> MPFVNKQFNYKDPVNGVDIAYIKIPNAGQMQPVKAFKIHNKIWVIPERDTFTNPEEGDLNPPPEAKQVPVSYYDSTYLSTDNEKDNYLKGVTKLFERIYSTDLGRMLLTSIVRGIPFWGGSTIDTELKVIDTNCINVIQPDGSYRSEELNLVIIGPSADIIQFECKSFGHEVLNLTRNGYGSTQYIRFSPDFTFGFEESLEVDTNPLLGAGKFATDPAVTLAHQLIHAGHRLYGIAINPNRVFKVNTNAYYEMSGLEVSFEELRTFGGHDAKFIDSLQENEFRLYYYNKFKDIASTLNKAKSIVGTTASLQYMKNVFKEKYLLSEDTSGKFSVDKLKFDKLYKMLTEIYTEDNFVKFFKVLNAKTFLNFDKAVFKINIVPKVNYTIYDGFNLRNTNLAANFNGQNTEINNMNFTKLKNFTGLFEFYKLLCVRGIITSKTKSLDKGYNKALNDLCIKVNNWDLFFSPSEDNFTNDLNKGEEITSDTNIEAAEENISLDLIQQYYLTFNFDNEPENISIENLSSDIIGQLELMPNIERFPNGKKYELDKYTMFHYLRAQEFEHGKSRIALTNSVNEALLNPSRVYTFFSSDYVKKVNKATEAAMFLGWVEQLVYDFTDETSEVSTTDKIADITIIIPYIGPALNIGNMLYKDDFVGALIFSGAVILLEFIPEIAIPVLGTFALVSYIANKVLTVQTIDNALSKRNEKWDEVYKYIVTNWLAKVNTQIDLIRKKMKEALENQAEATKAIINYQYNQYTEEEKNNINFNIDDLSSKLNESINKAMININKFLNQCSVSYLMNSMIPYGVKRLEDFDASLKDALLKYIYDNRGTLIGQVDRLKDKVNNTLSTDIPFQLSKYVDNQRLLSTFTEYIKNIINTSILNLRYESNHLIDLSRYASKINIGSKVNFDPIDKNQIQLFNLESSKIEVILKNAIVYNSMYENFSTSFWIRIPKYFNSISLNNEYTIINCMENNSGWKVSLNYGEIIWTLQDTQEIKQRVVFKYSQMINISDYINRWIFVTITNNRLNNSKIYINGRLIDQKPISNLGNIHASNNIMFKLDGCRDTHRYIWIKYFNLFDKELNEKEIKDLYDNQSNSGILKDFWGDYLQYDKPYYMLNLYDPNKYVDVNNVGIRGYMYLKGPRGSVMTTNIYLNSSLYRGTKFIIKKYASGNKDNIVRNNDRVYINVVVKNKEYRLATNASQAGVEKILSALEIPDVGNLSQVVVMKSKNDQGITNKCKMNLQDNNGNDIGFIGFHQFNNIAKLVASNWYNRQIERSSRTLGCSWEFIPVDDGWGERPL;> MKINNNFNIDSLIDNRDVAIVRGRKTDTFFKVFQVAPNIWVAPERYYGESLNINEDQKSDGGIYDSNFLLTNDEKDEFLQATVKILQRINNNVIGAKLLSLISTAIPFPYEYKPGDYRQTNYLVSKDNQHYYTANLVIFGPGTNIVENNAVYYKKEDSENGMGTMSEIWFQPFLTYKYDQFYVDPALELIKCLIKSLYYLYGIKPSDDLSIPYRLRSEFNSLEYSELDMVDFLISGGTDYKLLNTNPYWFTDNYFINAPKNFEKYKNDYETKIKNNNDIANSIKLYLEQKFKTNVQDIWELNLSYFSTEFEIMMPEIFNNALNHYHRKEYYVIDYFKNYNINGFINGQIKTILLLSKYNKNIINKPELIVNLINENNSVLMKSNIYGDGLKGTIGNFYAVYKIPYNIGDEYHINSSDSCLDNVDIKEIDNIPPINDADIYPYRKNCDPFTPVYNITETKEINTTIPFPVNYLQAQVTNSNDINLSSDFLKVISSKDRSLVYSFLDNTIDYLDSIKYDGPIDTDKKYYLWLKEIFRNYSFDMTETQEVNTLCGFNKVVPWLGKALNILNTGNSFIEEFKTLGPISLINKKENITMPKIEIDEIPNSMLNLSFKDLSENLFNIFSKNNSYFEKIYYDFLDQWWTQYYSQYFDLICMAKRSVLAQESLIKKIIQKKLSYLIGNSNISSDNLALMNLTTTNTLRDISNESQIAMNNVNNFLNNVAICVFQTNIYPKFISFMEQCINNINKNTREFIQKCTNITENEKLQLINQNIFSSLDFDFLNIENLKSLFNSETGLLIKEETSPYELVLYAFQEPGNNAIGDASGKNTSIEYSKDIGLVYGINSDALYLNGSNQSISFSNDFFENGLTNSFSIYFWLRNLGKDTIKSKLIGSKEDNCGWEIYFQDTGLVFNMIDSNGNEKNIYLSDVSNNSWHYITISVDRLKEQLLIFIDDNLVANESIKEILNIYSSNIISLLSENNPSYIEGLTILNKPTTSQEVLSNYFKVLNNSYIRDSSEERLEYNKTYQLYNYVFSENPIYEIKQNNNIYLTINNTNNLNLQVSKFKLLSINPNKQYVQKLDEVIISVLDNMEKYIDISEDNRLQLIDNKNNAKKMIISNDIFISNCLTLSYNGKYICLSMKDENHNWMICNNDMSKYLYLWSFK;> MNNLKPFIYYDWEKTILKNTKENYSINEIIPKTFFMELHGTKITNSTLNGTWKSWNLTNEGEGSYPVLKCIIDDGYLDMNFGASSEKIPLKNVWIKLCMKINPNSDGTYSIPEKSSSFYIKDNSLKISKDNLILDKYLNKLMLSYFKNNIKNIEMFINKSRIQTKVVGDLSLLGWNTENSVSFRTMNEFIKKDNLYPKDFKAVYSYRKMTFTATGTFDSWEMTTGADGRNIRFKCPIKYAVYDLDGDVFNSSTENFLLIQVDLTYFDSKTTINDPTGENDGKQFNLKIKTNDDKLKNVLIVTYNLTDTDGSMSSEDKDFLSLAFRNWFNENIQQFEQIFAYILLDETAKIPEYQWLKPTQISYGSASVETANDEPDLDASIFS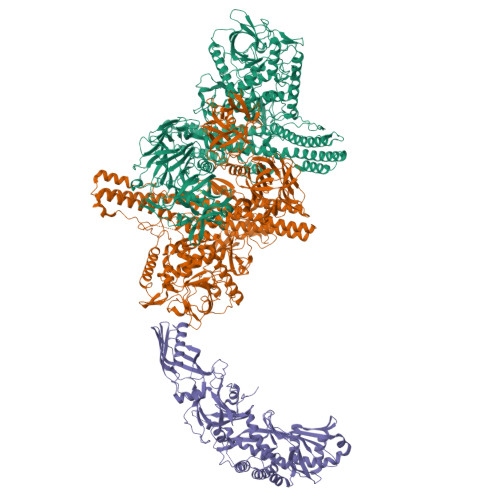AMSMVENNTNSTPSHAVDNRMLQLTKTQAAFGISFPLFIEHFLKQALLSSQFISVDDIVADINTLTITNNKQIIFGKVENSDGKNVDSSLKPGKLKLSLQNNLIVLELFDLTWEQGRGVTGHFDFRQEYELALESKSGKQIPILKVHDEPEIEYYVEEAQWKTNEDMIVSAVVGTVFSMILGASMKLAGSALSKAGKLIRSKATTIKGRKKIYINRSNVRQLRKDSGATEIELERINRRNSSIAAEDARLISNNGTTSIQTLGDMKKKPMSTGQRIAIGAKKIAGTAVMFGAVGLGMNFGEMLINYINAMENNDYSAIPGINSFMQQCIGAMQWPDKDSELKVTFGKLQGIYLLGGTLEKNNKTDNK> MGRGSHHHHHHGMASTRGVAKAVDFVPVESMETTMRSPVFTDNSSPPAVPQTFQVAHLHAPTGSGKSTKVPAAYAAQGYKVLVLNPSVAATLGFGVYMSKAHGIDPNIRTGVRAITTGGPITYSTYGKFLADGGCSGGAYDIIICDECHSTDSTSILGI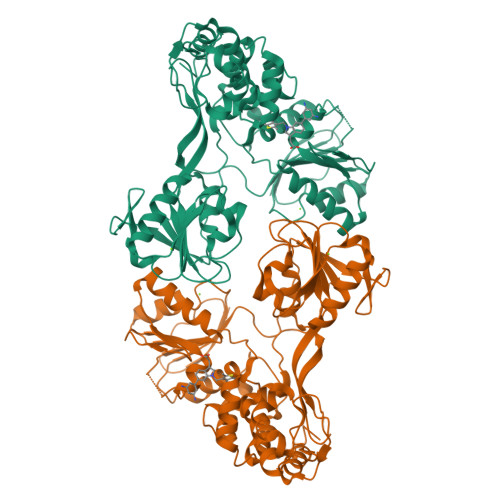GTVLDQAETAGARLVVLATATPPGSVTVPHPNIEEVALSNTGEIPFYGKAIPIEVIRGGRHLIFCHSKKKCDELAAKLSALGLNAVAYYRGLDVSVIPTSGDVVVVATDALMTGYTGDFDSVIDCNTCVTQTVDFSLDPTFTIDTTTVPQDAVSRSQRRGRTGRGRRGIYRFVTPGERPSGMFDSSVLCECYDAGCAWYELTPAETSVRLRAYLNTPGLPVCQDHLEFWESVFTGLTHIDAHFLSQTKQAGDNFPYLVAYQATVCARAQAPPPSWDQMWKSLTRLKPTLHGPTPLLYRLGALQNEVTLTHPVTKFIMACMSADLEVVTAAAREA>MNYPAEPFRIKSVETVSMIPRDERLKKMQEAGYNTFLLNSKDIYIDLLTDSGTNAMSDKQWAGMMMGDEAYAGSENFYHLERTVQELFGFKHIVPTHQGRGAENLLSQLAIKPGQYVAGNMYFTTTRYHQEKNGAVFVDIVRDEAHDAGLNIAFKGDIDLKKLQKLIDEKGAENIAYICLAVTVNLAGGQPVSMANMRAVRELTEAHGIKVFYDATRCVENAYFIKEQEQGFENKSIAEIVHEMFSYADGCTMSGKKD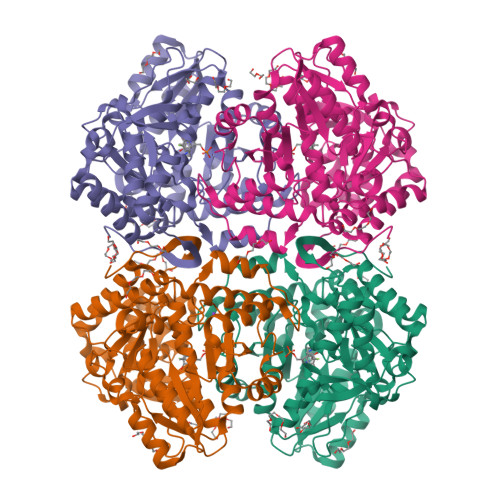CLVNIGGFLCMNDDEMFSSAKELVVVYEGMPSYGGLAGRDMEAMAIGLREAMQYEYIEHRVKQVRYLGDKLKAAGVPIVEPVGGHAVFLDARRFCEHLTQDEFPAQSLAASIYVETGVRSMERGIISAGRNNVTGEHHRPKLETVRLTIPRRVYTYAHMDVVADGIIKLYQHKEDIRGLKFIYEPKQLRHFTARFDYI[4x]>[2x]GCA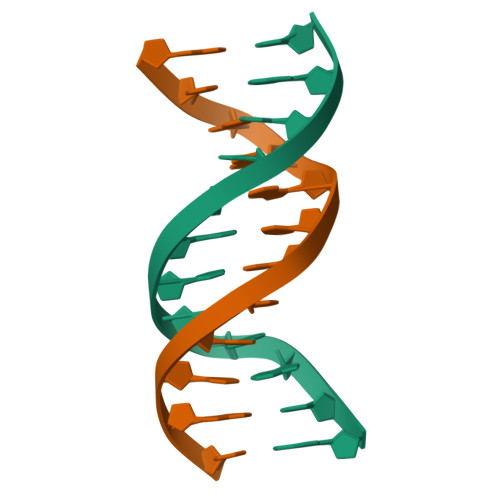AACGTTTGC>[2x]MSYNLLGFLQRSSNFQCQKLLWQLNGRLEYCLKDRMNFDIPEEIKQLQQFQKEDAALTIYEMLQNIFAIFRQDSSSTGWNETIVENLLANVYHQINHLKTVLEEKLEKEDFTR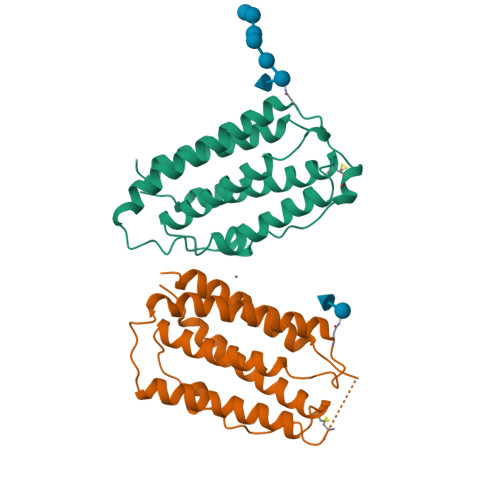GKLMSSLHLKRYYGRILHYLKAKEYSHCAWTIVRVEILRNFYFINRLTGYLRN>GPTPVEEAQQKTIEAITKAINYMAKRRIGALLTIERDTGMGDYIETGIPLNAKVSSELLINIFIPNTPLHDGAVIMKNNEIAAAACYLPLSESPFISKELGTRHRAAVGISEVTDSLTIIVSEETGGVSVAKNGDLHRELTEEALKEMLEAEF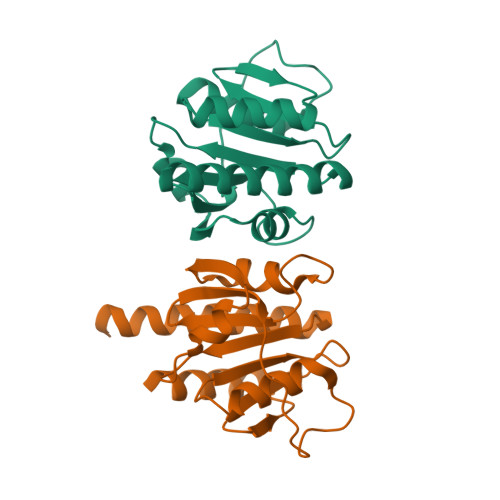K[2x]(2S)-2-(acetyloxy)-3-{[(R)-(2-aminoethoxy)(hydroxy)phosphoryl]oxy}propyl 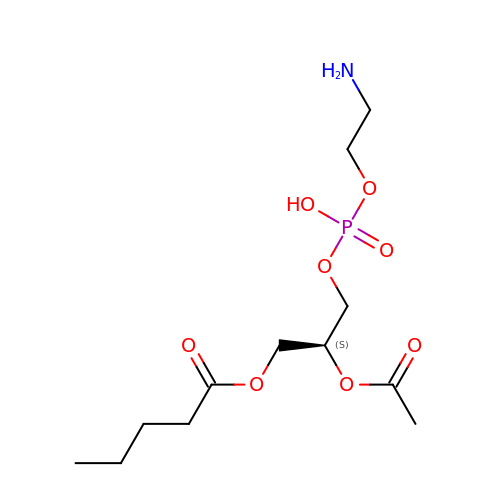pentanoate | C12 H24 N O8 P | PLBNSCVUDWCBFD-NSHDSACASA-N In siphophage T5, the unique RBP is located at the extremity of a central fiber. FhuA, an outer membrane E. coli iron-ferrichrome transporter, is the bacterial receptor recognized by T5 (25). We present the structures of T5 tail tip, determined by cryo–electron microscopy before and after interaction with its E. coli receptor, FhuA, reconstituted into nanodisc. These structures bring out the important conformational changes undergone by T5 tail tip upon infection, which include bending of T5 central fiber on the side of the tail tip, tail anchoring to the membrane, tail tube opening, and formation of a transmembrane channel.

Upon RBPpb5 binding to FhuA, the central fiber reorganizes: The three FNIIIs strings dissociate, two strings relocate on one side of BHPpb3, and the third one on the other side. This reorganization of the central fiber is allowed by the long linker that connects BHPpb3 hdIV to the first FNIII and which now runs perpendicular to the tail axis along BHPpb3. The central fiber bends by ~160° at the level of the hinge between the third pb4 FNIII and pb4 spike: The latter is now surrounded and stabilized by pb4 FNIIIs, which interact with and stabilize pb4 spike small decoration domains. pb4 spike also undergoes structural rearrangement, with a different twist of the spike. This bending and stabilization of the central fiber bring the tail tube closer to the membrane, orient it correctly, and anchor the tail to the membrane. Upon RBPpb5 binding to FhuA, a constraint at the RBPpb5-pb4 interface occurs, resulting in the different twist of pb4 spike observed in its proximal part. This twisting of the spike would pull on pb4 FNIII-spike linker, leading to the disruption of the FNIII-spike interaction network. The association between this FNIII and the spike is thus loosened; the pb4 FNIII-spike linker reorganizes and stabilizes a new interaction network between the three FNIII strings and the spike. This series of events results in the bending of the central fiber, at the level of the FNIII-spike hinge, on the side of the tube, pulling the tube toward the host membrane. The map after interaction with the receptor contains the spike decoration domains and the FNIIIs while that before interaction contains only pb4 spike.

>[3x]MKKILDSAKNYLNTHDKLKTACLIALELPSSSGSAATYIYLTDYFRDVTYNGILYRSGKVKSISSHKQNRQLSIGSLSFTITGTAEDEVLKLVQNGVSFLDRGITIHQAIINEEGNILPVDPDTDGPLLFFRGRITGGGIKDNVNTSGIGTSVITWNCSNQFYDFDRVNGRYTDDASHRGLEVVNGTLQPSNGAKRPEYQEDYGFFHSNKSTTILAKYQVKEERYKLQSKKKLFGLSRSYSLKKYYETVTKEVDLDFNLAAKFIPVVYGVQKIPGIPIFADTELNNPNIVYVVYAFAEGEIDGFLDFYIGDSPMICFDETDSDTRTCFGRKKIVGDTMHRLAAGTSTSQPSVHGQEYKYNDGNGDIRIWTFHGKPDQTAAQVLVDIAKKKGFYLQNQNGNGPEYWDSRYKLLDTAYAIVRFTINENRTEIPEISAEVQGKKVKVYNSDGTIKADKTSLNGIWQLMDYLTSDRYGADITLDQFPLQKVISEAKILDIIDESYQTSWQPYWRYVGWNDPLSENRQIVQLNTILDTSESVFKNVQGILESFGGAINNLSGEYRITVEKYSTNPLRINFLDTYGDLDLSDTTGRNKFNSVQASLVDPALSWKTNSITFYNSKFKEQDKGLDKKLQLSFANITNYYTARSYADRELKKSRYSRTLSFSVPYKFIGIEPNDPIAFTYERYGWKDKFFLVDEVENTRDGKINLVLQEYGEDVFINSEQVDNSGNDIPDISNNVLPPRDFKYTPTPGGVVGAIGKNGELSWLPSLTNNVVYYSIAHSGHVNPYIVQQLENNPNERMIQEIIGEPAGLAIFELRAVDINGRRSSPVTLSVDLNSAKNLSVVSNFRVVNTASGDVTEFVGPDVKLAWDKIPEEEIIPEIYYTLEIYDSQDRMLRSVRIEDVYTYDYLLTYNKADFALLNSGALGINRKLRFRIRAEGENGEQSVGWATI;>[3x]MISNNAPAKMVLNSVLTGYTLAYIQHSIYSDYDVIGRSFWLKEGSNVTRRDFTGIDTFSVTINNLKPTTTYEVQGAFYDSIIDSELLNAQIGINLSDKQTFKMKSAPRITGARCESEPVDVGVGAPIVYIDTTGEADYCTIELKDNSNANNPWVKYYVGALMPTIMFGGVPIGSYKVRISGQISLPDGVTIDSSGYYEYPNVFEVRYNFVPPAAPINIVFKAARIADGKERYDLRVQWDWNRGAGANVREFVLSYIDSAEFVRTGWTKAQKINVGAAQSATIISFPWKVEHKFKVSSIAWGPDAQDVTDSAVQTFILNESTPLDNSFVNETGIEVNYAYIKGKIKDGSTWKQTFLIDAATGAINIGLLDAEGKAPISFDPVKKIVNVDGSVITKTINAANFVMTNLTGQDNPAIYTQGKTWGDTKSGIWMGMDNVTAKPKLDIGNATQYIRYDGNILRISSEVVIGTPNGDIDIQTGIQGKQTVFIYIIGTSLPAKPTSPAYPPSGWSKTPPNRTSNTQNIYCSTGTLDPVTNQLVSGTSWSDVVQWSGTEGVDGRPGATGQRGPGMYSLAIANLTAWNDSQANSFFTSNFGSGPVKYDVLTEYKSGAPGTAFTRQWNGSAWTSPAMVLHGDMIVNGTVTASKIVANNAFLSQIGVNIIYDRAAALSSNPEGSYKMKIDLQNGYIHIR>[2x]MSSRYLLSPAAQAHLEEIWDCTYDRWGVDQAEQYLRELQHAIDRAAANPRIGRACDEIRPGYRKLSAGSHTLFYRVTGEGTIDVVRVLHQRMDVDRNL;>MGKNTSFVLDEHYSAFIDGEIA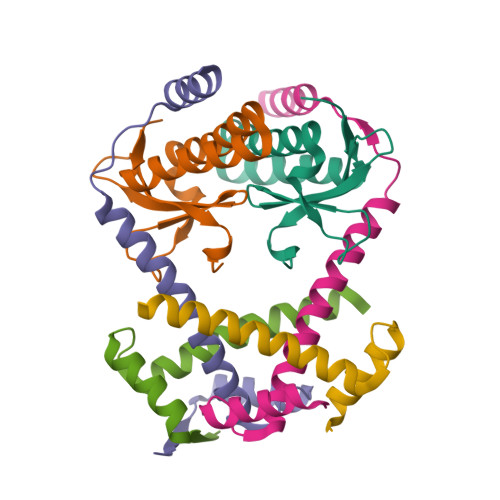AGRYRSASEVIRSALRLLEDRETQLRALREALEAGERSGSSTPFDFDGFLGRKRADASRGR[4x]In coumarin biosynthesis, a BAHD acyltransferase-family enzyme COSY was recently discovered to accelerate coumarin formation as the only known BAHD enzyme to catalyze an intramolecular acyl transfer reaction. To understand the mechanistic basis for the unconventional activity of COSY as a BAHD-family enzyme, we present several crystal structures of A. thaliana COSY (AtCOSY) in its apo and various ligand-bound forms. The AtCOSY active site is located at the interface between the two pseudo-symmetric domains, and features the conserved catalytic residues, His161 and Trp371, stemming from the N- and C-terminal domains, respectively.

We noticed that a single oxidation of Cys308 to sulfenic acid was present in the CoA-bound structure, suggesting that it may play a role as a redox-gate for the proper substrate entry. Moreover, based on our observation of Cys308 oxidation in the CoA-bound structure, we generated the C308A and C308S mutants, and assayed their activities in buffers containing a concentration gradient of hydrogen peroxide. Even so, varying redox environments had little effect on coumarin synthase activity for wild-type (WT), C308A, and C308S enzymes. Thus, C308 oxidation is likely a crystallography artifact in our solved structures. Guided by both the CoA-bound and scopoletin-bound AtCOSY structures, we modeled the trans-6OHFCoA substrate in the COSY active site. This reconstructed pose of trans-6OHFCoA indicates that residues Phe40, Tyr42, His161, Cys164, and Trp371 engage close contacts with the substrate, and are likely involved in specific substrate binding and catalysis. Indeed, we observed conformational differences of an active-site loop containing Tyr373 and Leu374 between the CoA-bound and scopoletin-bound AtCOSY structures. In the CoA-bound structure, Tyr373 exhibits π-π stacking interaction with the adenine portion of CoA causing Leu374 to shift towards C2 of 6OHFCoA, relative to its conformation in the scopoletin-bound structure. The Y373A and Y373F mutants exhibit WT-level coumarin synthase activities, whereas the L374A mutant shows a significant decrease in activity similar to that of the W371A mutant. These observations indicate that the π-π stacking interaction of Tyr373 with CoA does not contribute significantly to the coumarin synthase activity, while Leu374 on this dynamic loop region is likely involved in catalysis, albeit in a nonessential manner.

> MATLEITDIALVQPSHQPLSNDQTLSLSHLDNDNNLHVSFRYLRVYSSSSSTVAGESPSAVVSASLATALVHYYPLAGSLRRSASDNRFELLCSAGQSVPLVNATVNCTLESVGYLDGPDPGFVERLVPDPTREEGMVNPCILQVTMFQCGGWVLGASIHHAICDGLGASLFFNAMAELARGATKISIEPVWDRERLLGPREKPWVGAPVRDFLSLDKDFDPYGQAIGDVKRDCFFVTDDSLDQLKAQLLEKSGLNFTTFEALGAYIWRAKVRAAKTEEKENVKFVYSINIRRLMNPPLPKGYWGNGCVPMYAQIKAGELIEQPIWKTAELIKQSKSNTSDEYVRSFIDFQELHHKDGINAGTGVTGFTDWRYLGHSTIDFGWGGPVTVLPLSNKLLGSMEPCFFLPYSTDAAAGSKKDSGFKVLVNLRESAMPEFKEAMDKFHKGEFALS>[2x]SNVPHKSSLPEGIRPSTVLRIRGLVPPNASRFHVNLLCGEEQGSDAALHFNPRLDTSEVVFNSKEQGSWGREERGPGVPFQRGQPFEVLIIASDDGFKAVVG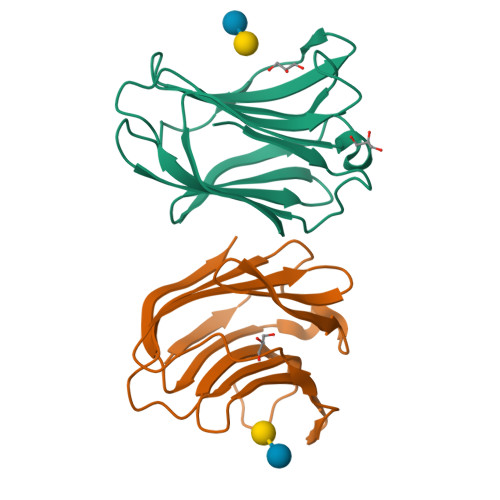DAQYHHFRHRLPLARVRLVEVGGDVQLDSVRIF> MKKANEALTRNRELTTVLVKNLPKSYNQNKVYKYFKHCGPIIHVDVADSLKKNFRFARIEFARYDGALAAITKTHKVVGQNEIIVSHLTECTLWMTNFPPSYTQRNIRDLLQDINVVALSIRLPSLRFNTSRRFAYIDVTSKEDARYCVEKLNGLKIEGYTLVTKVSNPLEKSKRTDSATLEGREIMIRNLSTELLDENLLRESFEGFGSIEKINIPAGQKEHSFNNCCAFMVFENKDSAERALQMNRSLLGNREISVSLADKKPFLERNEVKRLLASRNSKELETLICLFPLSDKVSPSLICQFLQEEIHINEKDIRKILLVSDFNGAIIIFRDSKFAAKMLMILNGSQFQGKVIRSGTINDMKRYYNNQQNHSMKHVKPSCINMMEKGPNLQVKKKIPDKQEQMSNDDFRKMFLGEHHHHHH;> MLFFSFFKTLVDQEVVVELKNDIEIKGTLQSVDQFLNLKLDNISCTDEKKYPHLGSVRNIFIRGSTVRYVYLNKNMVDTNLLQDATRREVMTERK;> METPLDLLKLNLDERVYIKLRGARTLVGTLQAFDSHCNIVLSDAVETIYQLNNEELSESERRCEMVFIRGDTVTLISTPSE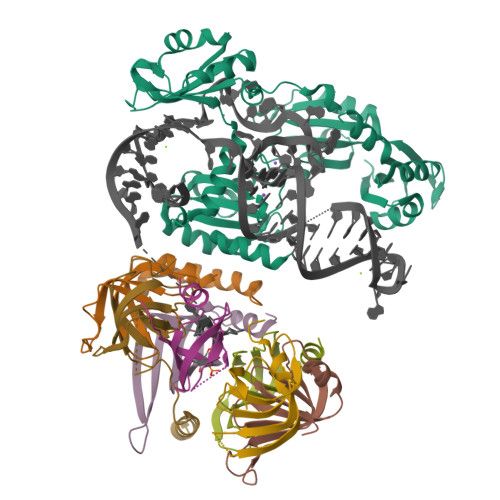DDDGAVEIWSHPQFEK;> MLPLYLLTNAKGQQMQIELKNGEIIQGILTNVDNWMNLTLSNVTEYSEESAINSEDNAESSKAVKLNEIYIRGTFIKFIKLQDNIIDKVKQQI;> MSLPEILPLEVIDKTINQKVLIVLQSNREFEGTLVGFDDFVNVILEDAVEWLIDPEDESRNEKVMQHHGRMLLSGNNIAILVPGGKKTPTEAL;> GSMSGKASTEGSVTTEFLSDIIGKTVNVKLASGLLYSGRLESIDGFMNVALSSATEHYESNNNKLLNKFNSDVFLRGTQVMYISEQKI;> MHQQHSKSENKPQQQRKKFEGPKREAILDLAKYKDSKIRVKLMGGKLVIGVLKGYDQLMNLVLDDTVEYMSNPDDENNTELISKNARKLGLTVIRGTILVSLSSAEGSDVLYMQK;> MSATLKDYLNKRVVIIKVDGECLIASLNGFDKNTNLFITNVFNRISKEFICKAQLLRGSEIALVGLIDAENDDSLAPIDEKKVPMLKDTKNKIENEHVIWEKVYESKTKHHHHHH>APQTITELCSEYHNTQIYTINDKILSYTESMAGKREMVIITFKSGETFQVEVPGSQHIDSQK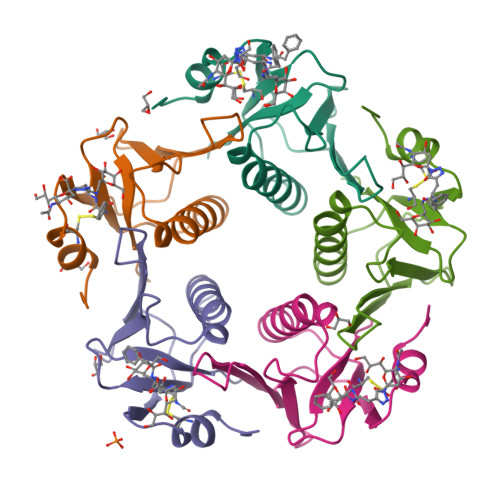KAIERMKDTLRITYLTETKIDKLCVWNNKTPNSIAAISMKN[5x]>[5x]DYKDDDDKLHSQANLMRLKSDLFNRSPMYPGPTKDDPLTVTLGFTLQDIVKADSSTNEVDLVYYEQQRWKLNSLMWDPNEYGNITDFRTSAADIWTPDITAYSSTRPVQVLSPQIAVVTHDGSVMFIPAQRLSFMCDPTGVDSEEGATCAVKFGSWVYSGFEIDLKTDTDQVDLSSYYASSKYEILSATQTRQVQHYSCCPEPYIDVNLVVKFRE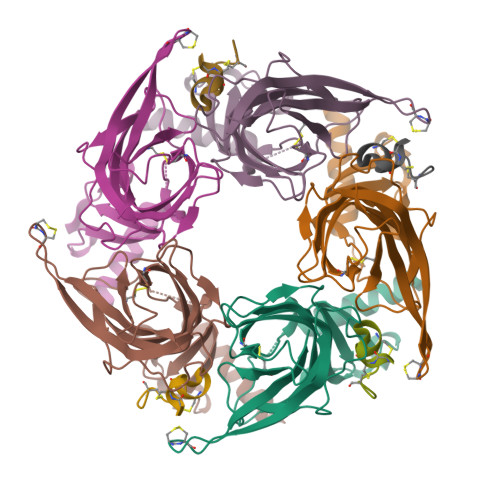RRAGNGFFRNLFDSR;>[4x]GCCSHPACSVNHPELCX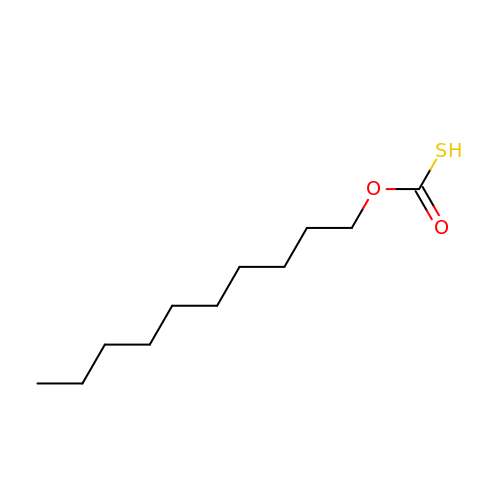O-DECYL HYDROGEN THIOCARBONATE | C11 H22 O2 S | RFWUWWWJCLPVPT-UHFFFAOYSA-N N-[(1S)-1-cyclopropylethyl]-2-phenoxy-5H-pyrrolo[2,3-b]pyrazine-7-carboxamide | C18 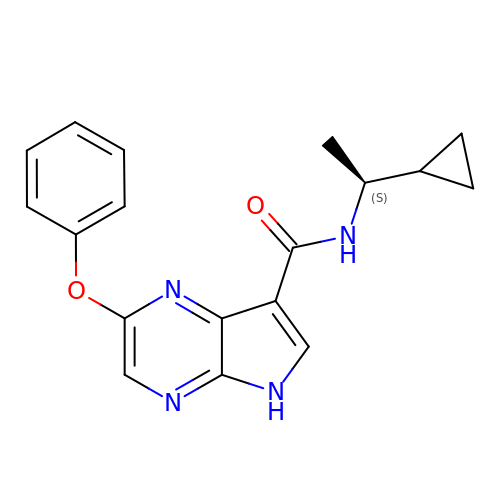H18 N4 O2 | TUNBOTWJAARGCJ-NSHDSACASA-N>[2x]MKLERVTVKNFRSHSDTVVEFKEGINLIIGQNGSGKSSLLDAILVGLYWPLRIKDIKKDEFTKVGARDTYIDLIFEKDGT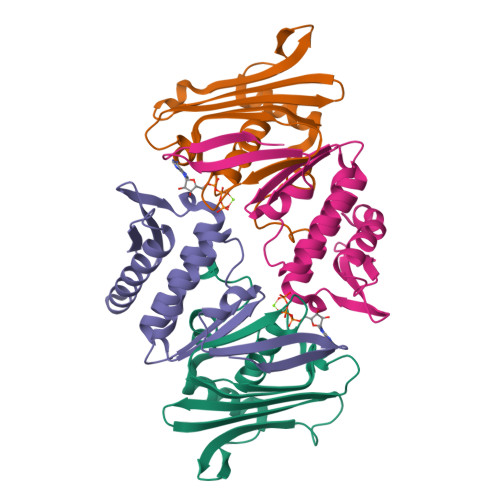KYRITRRFLKGYSSGEIHAMKRLVGNEWKHVTEPSSKAISAFMEKLIPYNIFLNAIYIRQGQIDAILES;>[2x]KYKALAREAALSKIGELASEIFAEFTEGKYSEVVVRAEENKVRLFVVWEGKERPLTFLSGGERIALGLAFRLAMSLYLAGEISLLILDEPTPYLDEERRRKLITIMERYLKKIPQVILVSHDEELKDAADHVIRISLENGSSKVEVVS> DACEQAAIQCVESACESLCTEGEDRTGCY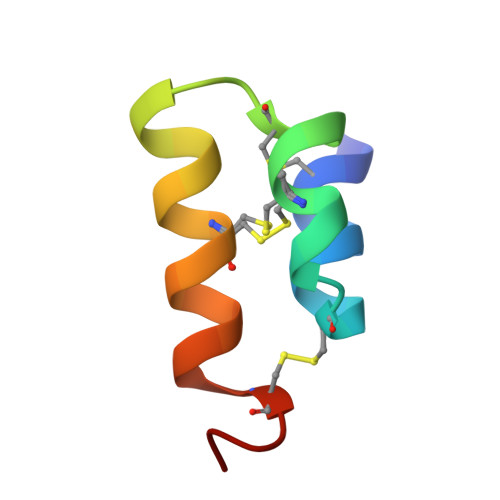MYIYSNCPPYV> MTLSLWKREQARLKAHVVDRDTEAWQRDPAFSGLQRVGGVDVSFVKGDSVRACASLVVLSFPELEVVYEESRMVSLTAPYVSGFLAFREVPFLLELVQQLREKEPGLMPQVLLVDGNGVLHHRGFGVACHLGVLTDLPCVGVAKKLLQVDGLENNALHKEKIRLLQTRGDSFPLLGDSGTVLGMALRSHDR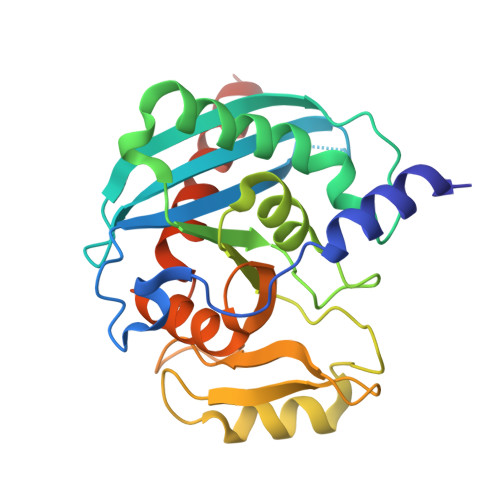STRPLYISVGHRMSLEAAVRLTCCCCRFRIPEPVRQADICSREHIRKSAAALEHHHHHH>GQTVSSESTEELDDASKVINYYHMSLAVLRHVANAKDINAVLGYMEQTGKVPEVDPIAPPEIAARDTAELLDPGDYFNPEVRQNLKQNYAGLFNVRTQFYDNFNKFLAYKKSKDTAKTAQLLDENYKLSVELSEYKQVIFDILSPLTEQAESELLADEPLKDQIM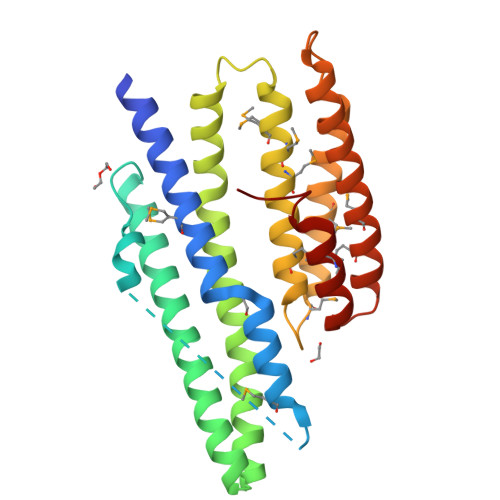AMRKMSGTVQSIMNLYSRKHAMDGVRIDLKMAELEKELKAAEKIPAVTGYDEELKNFQSFLSTVKSFMNDMQKARSKGAYSDKEYQAMSEAYEYGLSVI[2x]> SWQ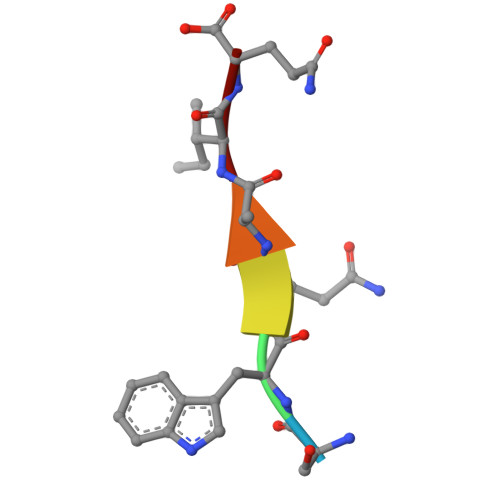AIQ>[4x]MNNNDIEYNAPSEIKYIDVVNTYDLEEEASKVVPHGGFNYIAGASGDEWTKRANDRAW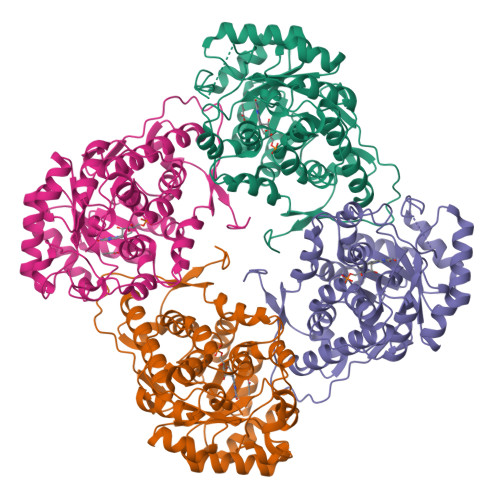KHKLLYPRLAQDVEAPDTSTEILGHKIKAPFIMAPIAAHGLAHTTKEAGTARAVSEFGTIMSISAYSGATFEEISEGLNGGPRWFQIYMAKDDQQNRDILDEAKSDGATAIILTADSTVSGNRDRDVKNKFVYPFGMPIVQRYLRGTAEGMSLNNIYGASKQKISPRDIEEIAGHSGLPVFVKGIQHPEDADMAIKRGASGIWVSNHGARQLYEAPGSFDTLPAIAERVNKRVPIVFDSGVRRGEHVAKALASGADVVALGRPVLFGLALGGWQGAYSVLDYFQKDLTRVMQLTGSQNVEDLKGLDLFDNPYGYEY>[2x]SKEYHIDEEVGFALPNPQENLPDFYNDWMFIAKHLPDLIESGQLRERVEKLNMLSIDHLTDHKSQRLARLVLGCITMAYVWGKGHGDVRKVLPRNIAVPYCQLSKKLELPPILVYADCVLANWKKKDPNKPLTYENMDVLFSFRDGDCSKGFFLVSLLVEIAAASAIKVIPTVFKAMQMQERDTLLKALLEIASCLEKALQVFHQIHDH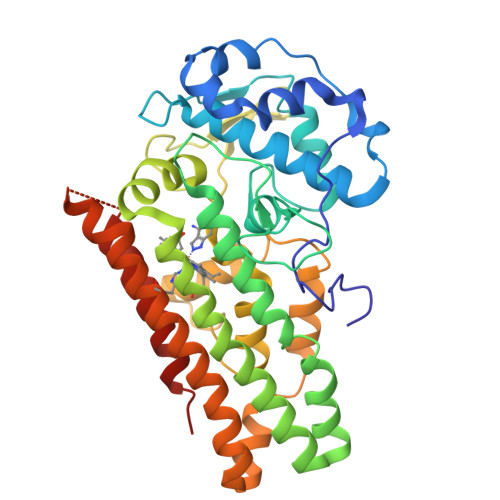VNPKAFFSVLRIYLSGWKGNPQLSDGLVYEGFWEDPKEFAGGSAGQSSVFQCFDVLLGIQQTAGGGHAAQFLQDMRRYMPPAHRNFLCSLESNPSVREFVLSKGDAGLREAYDACVKALVSLRSYHLQIVTKYILIPASQQPKENKTSEDPSKLEAKGTGGTDLMNFLKTVRSTTEKSLLKEG methyl 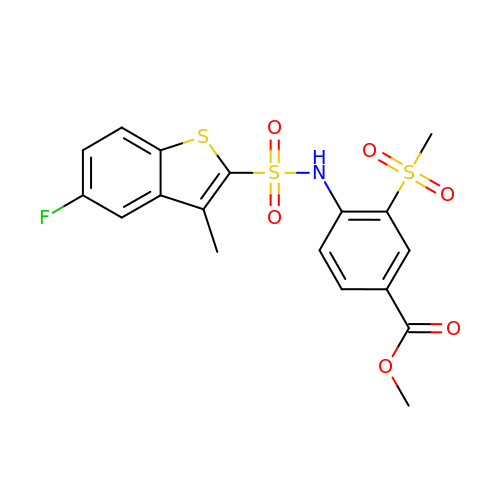4-(5-fluoro-3-methyl-1-benzothiophene-2-sulfonamido)-3-(methanesulfonyl)benzoate | C18 H16 F N O6 S3 | HQGLOZAWIWWMET-UHFFFAOYSA-N>[4x]MHHHHHHMARIRAMKRHYEAVVIGGGIIGSAIAYYLAKENKNTALFESGTMGGRTTSAAAGMLGAHAECEERDAFFDFAMHSQRLYKGLGEELYALSGVDIRQHNGGMFKLAFSEEDVLQLRQMDDLDSVSWYSKEEVLEKEPYASGDIFGASFIQDDVHVEPYFVCKAYVKAAKMLGAEIFEHTPVLHVERDGEALFIKTPSGDVWANHV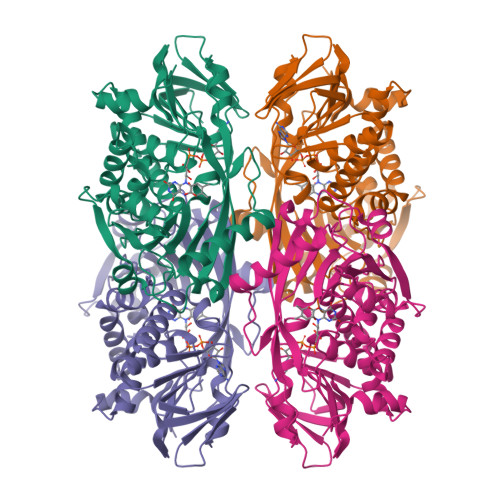VVASGVWSGMFFKQLGLNNAFLPVKGECLSVWNDDIPLTKTLYHDHCYIVPRKSGRLVVGATMKPGDWSETPDLGGLESVMKKAKTMLPAIQNMKVDRFWAGLRPGTKDGKPYIGRHPEDSRILFAAGHFRNGILLAPATGALISDLIMNKEVNQDWLHAFRIDRKEAVNI> MASWDSPTASSNGDLIEEIQASSTSTDPRTFTGLSIVEDIGDVVPVTDNASPALPVSLTDADGNDVVVEDVSRILPLDLYGTYSKTIAGLGLVDNIVGRTVSSTEPALADTEVVTTGGHTLNAEAILNLHPTLVIIDHSIGPREVIDQIRAAGVATVIMSPQRSIASIGDDIRDIASVVGLPEEGEKLAERSVAEVEEASTVVDELTPEDPLKMVFLYAAGTGGVFFILGDAYGGRDLIEGLGGVDMAAEKGIMDLAPANAEALAELNPDVFVMMSEGLVSTGGIDGLMERPGIAQTTAGQNQRVLALPDGQSLAFGAQTGELLLRASRELYVQGGELEHHHHHH

HmuTUV forms an ABC-type heme transporter system, in which HmuT, HmuU, and HmuV are the heme binding lipoprotein, permease, and ATPase, respectively. CgHmuT consists of two lobes connected with a α-helix, both of which consist of a five-stranded β-sheet and four α-helices. His141 and Tyr240 are coordinated to the heme as the axial ligands and Arg242 forms a hydrogen bond with Tyr240 in CgHmuT. As CgHmuT is a substrate (heme) binding protein that shuttles heme to the cognate ABC-type heme transporter CgHmuUV in Corynebacteria, the regulation of heme binding and release is very important for its physiological function.

The purified heme-bound proteins were crystallized, and the crystal structures of H141A-, Y240A-, and R242A-CgHmuT were determined in the holo-form at the resolution of 1.30, 1.65, and 1.30 Å, respectively. While two different orientations of heme were observed in Y240A-CgHmuT, heme was accommodated with a single orientation in H140A- and R242A-CgHmuT. Ferric R242A-CgHmuT showed the ν2 bands at 1556 and 1581 cm−1 and the ν3 bands at 1476 and 1503 cm−1, which were identical to those of the wild type. The set of the ν2 and ν3 bands at 1556 and 1476 cm−1 are due to a high-spin heme, while those at 1581 and 1503 cm−1 are due to a low-spin heme. These results indicate that there is equilibrium between the high-spin and low-spin species in the R242A-CgHmuT solution, as is the case of the wild type. While the heme bound to wild-type CgHmuT is not reduced by dithionite under normal conditions, the heme in H141A-, Y240A-, and R242A-CgHmuT are reduced by dithionite. The change in the redox property of R242A-CgHmuTA will be caused by a similar effect upon a loss of hydrogen bond between Tyr240 and Arg242.> MTVTIEIKKKPQIKYEEKQAVMPESAAGTYTFEVQTIDGKLDYEPYFTSSTLPWITGAPTISSRTDPNKDVISFTCLKNKTVWNRRAYIKFKDKKTGQYIKGADGKADLTVNIIQKKNENPVVHYKWVDGIGAPTENQKIKMKIKNNGIETEDYFTDPFVFKWKETADTKFYNVRKLDKLYVQGQFPSNYFVINGIRNEQIQ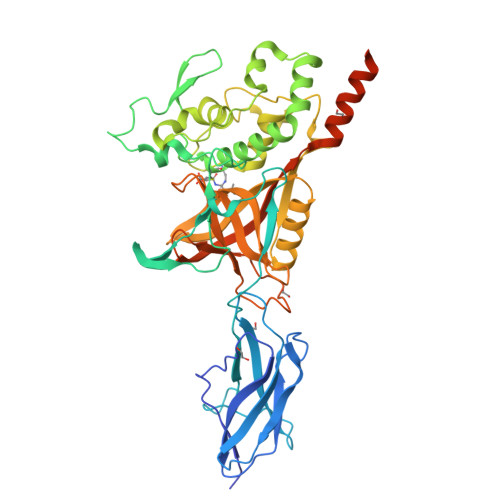GRDISQCWAKTASNMLHWWFEQNKDYIEQYKQKAAIEEWKRPLYKHDYIRGLQDEDEGKKSNIANIFRAYSHNNARGGYIEDGLTWYLYKRDGQKNLGSIYPGLFNDVFAHDTSPINIERCETKKEFEQLMNKTLDNKRAIGIFWQGSKGNRPYQHAVTCWGAAYDEDNNIICLYIAESNLPEAVLYPFGVRYKGNIYEEAEKNRTYMFNYALSKPENIYIDGLTTLDKGEDQWKKWLEAHQKGELNSKLEGKPIPNPLLGLDSTRTGHHHHHH> TDTTNSIKHVISPLARQTLQDRDLTRPVAGKRPIRLLPWLQVVKIGGRVMDRGADAILPLVEELRKLLPEHRLLILTGAGVRARHVFSVGLDLGLPVGSLAPLAASEAGQNGHILAAMLASEGVSYVEHPTVADQLAIHLSATRAVVGSAFPPYHHHEFPGSRIPPHRADTGAFLLADAFGAAGLTIVENVDGIYTADPNGPDRGQARFLPETSATDLAKSEGPLPVDRALLDVMATARHIERVQVVNGLVPGRLTAALRGEHVGTLIRTGVRPA;> ANSTAELEELLMQRSLTDPQLQAAAAAAADFRILPDATVISIGGQSVIDRGRAAVYPLVDEIVAARKNHKLLIGTGAGTRARHLYSIAAGLGLPAGVLAQLGSSVADQNAAMLGQLLAKHGIPVVGGAGLSAVPLSLAEVNAVVFSGMPPYKLWMRPAAEGVIPPYRTDAGCFLLAEQFGCKQMIFVKDEDGLYTANPKTSKDAT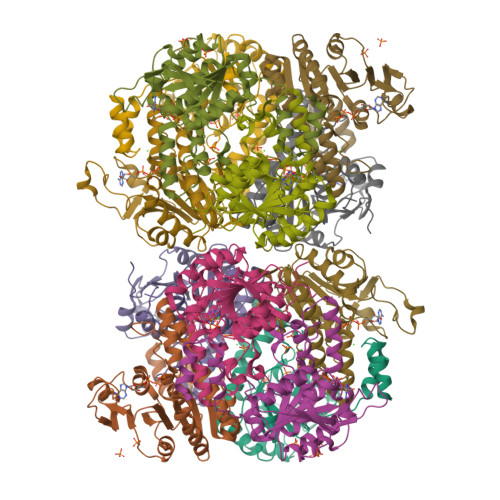FIPRISVDEMKAKGLHDSILEFPVLDLLQSAQHVREVQVVNGLVPGNLTRALAGEHVGTIITAS SNARE (soluble N-ethylmaleimide-sensitive factor (NSF) attachment protein receptor) proteins drive membrane fusion at different cell compartments as their core domains zipper into a parallel four-helix bundle. After fusion, these bundles are disassembled by the AAA+ (ATPase associated with diverse cellular activities) protein Sec18/NSF and its adaptor Sec17/α-SNAP to make them available for subsequent rounds of membrane fusion. The disassembly requires multiple ATP hydrolysis events in the presence of Mg2+; as few as six ATP hydrolysis events are sufficient. The side-loading and side-release mechanism explains how Sec18/NSF can disassemble SNAREs with constrained topologies.

We chose the Sso1–Sec9–Snc1/Snc2 complex (referred to as the ySNARE complex) because each component of this complex crosslinked with high confidence to the D2 domain of Sec18 (Snc1 is highly homologous to Snc2). We prepared the y20S complex in a nonhydrolyzing condition and, after single-particle cryo-EM data collection and processing, we obtained 381,591 high-quality particles that yielded eight three-dimensional (3D) classes into which models were built. In the structures of all eight classes, Sso1 is threaded through the D1 pore of Sec18. A characteristic phenylalanine side-chain density in Sso1 is present at the same position relative to Sec18 in all classes, allowing for reliable indexing of Sso1. The nucleotide states and the arrangements of D1 around the substrate were also the same among all eight classes, with the ADP-engaged E protomer forming the top of a spiral staircase of tyrosine residues. Protomers D, B and C were all ATP bound and formed the middle of the staircase. The bottom protomer, A, formed the base of the staircase. Protomer F, with no apparent density for nucleotide in D1, was not associated with Sso1. Given that this charge distribution is replicated between each pair of D2 subdomains around the D2 surface, it is unsurprising that the Habc domain adopts multiple corresponding rotational states over the eight classes, presumably because of the flexible linker that follows it.

>[6x]GAHMFKIPGFGKAAANHTPPDMTNMDTRTRHLKVSNCPNNSYALANVAAVSPNDFPNNIYIIIDNLFVFTTRHSNDIPPGTIGFNGNQRTWGGWSLNQDVQAKAFDLFKYSGKQSYLGSIDIDISFRARGKAVSTVFDQDELAKQFVRCYESQIFSPTQYLIMEFQGHFFDLKIRNVQAIDLGDIEPTSAVATGIETKGILTKQTQINFFKGRDGLVNLKSSNSLRPRSNAVIRPDFKFEDLGVGGLDKEFTKIFRRAFASRIFPPSVIEKLGISHVKGLLLYGPPGTGKTLIARKIGTMLNAKEPKIVNGPEILSKYVGSSEENIRNLFKDAEAEYRAKGEESSLHIIIFDELDSVFKQRGSRGDGTGVGDNVVNQLLAKMDGVDQLNNILVIGMTNRKDLIDSALLRPGRFEVQVEIHLPDEKGRLQIFDIQTKKMRENNMMSDDVNLAELAALTKNFSGAEIEGLVKSASSFAINKTVNIGKGATKLNTKDIAKLKVTREDFLNALNDVTPAFGISEEDLKTCVEGGMMLYSERVNSILKNGARYVRQVRESDKSRLVSLLIHGPAGSGKTALAAEIALKSGFPFIRLISPNELSGMSESAKIAYIDNTFRDAYKSPLNILVIDSLETLVDWVPIGPRFSNNILQMLKVALKRKPPQDRRLLIMTTTSAYSVLQQMDILSCFDNEIAVPNMTNLDELNNVMIESNFLDDAGRVKVINELSRSCPNFNVGIKKTLTNIETARHDEDPVNELVELMTQSA;>[3x]GMSDPVELLKRAEKKGVPSSGFMKLFSGSDSYKFEEAADLCVQAATIYRLRKELNLAGDSFLKAADYQKKAGNEDEAGNTYVEAYKCFKSGGNSVNAVDSLENAIQIFTHRGQFRRGANFKFELGEILENDLHDYAKAIDCYELAGEWYAQDQSVALSNKCFIKCADLKALDGQYIEASDIYSKLIKSSMGNRLSQWSLKDYFLKKGLCQLAATDAVAAARTLQEGQSEDPNFADSRESNFLKSLIDAVNEGDSEQLSEHCKEFDNFMRLDKWKITILNKIKESIQQQEDDLL;> GASHMSSSTPFDPYALSEHDEERPQNVQSKSRTAELQAEIDDTVGIMRDNINKVAERGERLTSIEDKADNLAVSAQGFKRGANRVRKAMWYKDLKMK;> GASHMSYNNPYQLETPFEESYELDEGSSAIGAEGHDFVGFMNKISQINRDLDKYDHTINQVDSLHKRLLTEVNEEQASHLRHSLDNFVAQATDLQFKLKNEIKSAQRDGIHDTNKQAQAENSRQRFLKLIQDYRIVDSNYKEENKEQAKRQYMIIQPEATEDEVEAAISDVGGQQIFSQALLNANRRGEAKTALAEVQARHQELLKLEKSMAELTQLFNDMEELVIEQQENVDVIDKNVEDAQLDVEQGVGHTDKAVKSARKARKNKIR;> GASHIKFTKQSSVASTRNTLKMAQDAERAGMNTLGMLGHQSEQLNNVEGNLDLMKVQNKVADEKVAELKKLNRSILAVHVSNPFNSKRRRREREEQLKNRKIEEKLMREQTSQQLSQSTQRIEGAMNANNNISEVRERYQRKNVLEKAKRYQFENDEEDDEMELEIDRNLDQIQQVSNRLKKMALTTGKELDSQQKRLNNIEESTDDLDINLHMNTNRLAGI>[2x]FTDEYQLFEELGKGAFSVVRRCMKIPTGQEYAAKIINTKKLSARDHQKLEREARICRLLKHPNIVRLHDSISEEGFHYLVFDLVTGGELFEDIVAREYYSEADASHCIQQILESVNHCHLNGIVHRDLKPENLLLASKSKGAAVKLADFGLAIEVQGDQQAWFGFAGTPGYLSPEVLRKD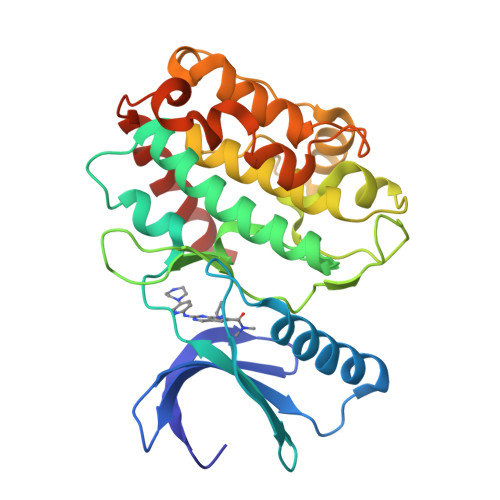PYGKPVDMWACGVILYILLVGYPPFWDEDQHRLYQQIKAGAYDFPSPEWDTVTPEAKDLINKMLTINPAKRITASEALKHPWICQRSTVASMMHRQETVDCLKKFNARRKLKGAILTTML>MKIERKFTTAEGGAYGGVGFTTTVSEIRNPDGTVVFRNESVEVPEGWSQVASDVLAQKYFRKAGVPARLKRVKEKGVPDFLWRSVPDEAELAKLPAAARFVGETSARQVFDRLAGAWAYWGWKGGYFSTEADARAYYDEMRHMLARQMAAPNSPQWFNTGLHWAYGIDGPSQGHFYVDHATGKLQKSDSAYEHPQPHACFIQSVQDDLVNEGGIMDLWVREARLFKYGSGTGTNFSSLRGEGEKLSGGGKSSGLMGFLKIGDRAAGAIKSGGTTRRAAKMVICDMDHPDIEQFINWKVIEEQKVASLVAGSKQHEAKLNDIFAAIRSFDGSIEGATDPAGNAGLKTAIRAAKKAMIPETYINRVLQYARQGFSSIEFPTYDTDWDSEAYTTVSGQNSNNSVRVTDAFLQAVKDDADWALVRRTDGKVAKTIKARELWDQVGHAAWACADPGIQFHDTVNAWHTCPEDGQIRGSNPCSEYMFLDDTACNLASMNLLTFFEAGRFDAEGYVHATRLWTVTLEISVMMAQFPSKEIAQLSYDFRTLGLGYANIGGLLMNMGLGYDSSEGRALCGALSAIMTGVAYATSAEMAGELGAFSGYERNAGHMLRVIRNHRTAAHGHTTGYEGVNVSPVALDQVNCPDPRLVALAKSSWDEALRLGEAHGYRNAQVTVIAPTGTIGLVMDCDTTGIEPDFALVKFKKLAGGGYFKIINRSVPAALETLGYASAQISQIVAYAVGHGTLANCPTISHSALVGHGFGAREIEKIEAALPSAFDIRFVFNQWTLGEDFCKGALGIPADKLADPTFDLLRHLGFTRAQIEAANDHVCGTMTLEGAPHLKAEHLPVFDCANPCGKKGKRYLSVESHIH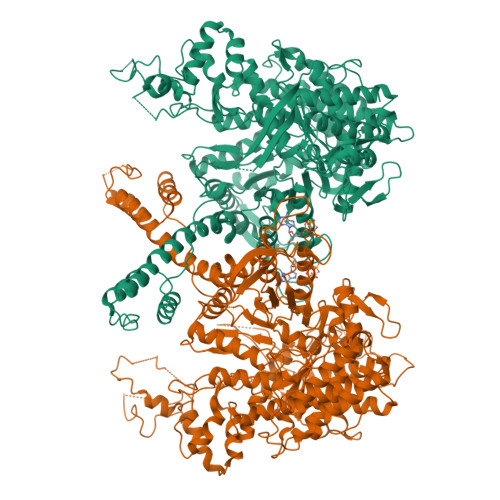MMAAAQSFISGAISKTINMPNSATIAETLAAYELSHSLGIKANALYRDGSKLSQPLASAL[2x]> SAAWEDEDLDTDNDNIPDAYEKNGYTIKDSIAVKWNDSFAEQGYKKYVSSYLESNTAGDPYTDYQKASGSIDKAIKLEARDPLVAAYPVVGVGMENLIISTNEHASSDQGKTVSRATTNSKTDANTVGVSISAGYQNGFTGNITTSYSHTTDNSTAVQDSNGESWNTGLSINKGESAYINANVRYYNTGTAPMYKVTPTTNLVLDGETLATIKAQDNQIGNNLSPNETYPKKGLSPLALNTMDQFNARLIPINYDQLKKLDSGKQIKLETTQVSGNYGTKNSQGQIITEGNSWSNYISQIDSVSASIILDTGSQTFERRVAAKEQGNPEDKTPEITIGEAIKKAFSATKNGELLYFNGIPIDESCVELIFDDNTSEIIKEQLKYLDDKKIYNVKLERGMNILIKVPSYFTNFDEYNNFPASWSNIDTKNQDGLQSVANKLSGETKIIIPMSKLKPYKRYVFSGYSKDPSTSNSITVNIKSKEQKTDYLVPEKDYTKFSYEFETTGKDSSDIEITLTSSGVIFLDNLSITELNSTPEILKEPEIKVPSDQEILDAHNKYYADIKLDTNTGNTYIDGIYFEPTQTNKEALDYIQKYRVEATLQYSGFKDIGTKDKEIRNYLG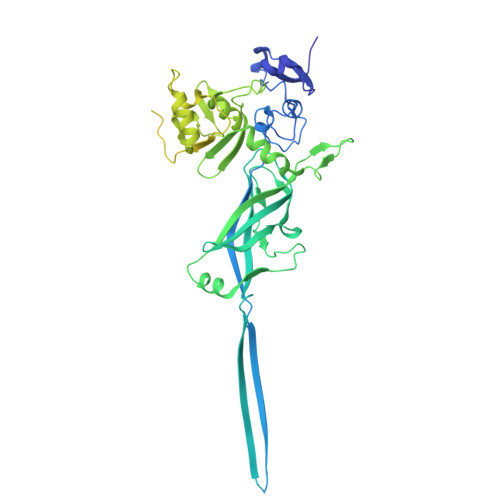DQNQPKTNYINFRSYFTSGENVMTYKKLRIYAVTPDNRELLVLSVN>GGAGGGGAACUUCUAUCUGGUGAUAGACGGGAACUCUAAAUUCCUUGAAAUGCCUCGCCGCAUUGGGUUCGAUUCCC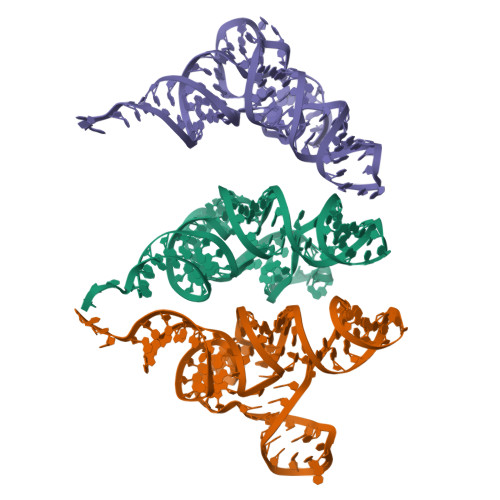UUCCCCUCCGCCA[3x]(2~{R},4~{S},5~{R},6~{R})-5-acetamido-2-[4-[(2~{R})-3-[2-[(2~{S},3~{R},4~{R},5~{R},6~{R})-6-(hydroxymethyl)-3,4,5-tris(oxidanyl)oxan-2-yl]ethylamino]-3-oxidanylidene-2-(2-phenylethanoylamino)propyl]-1,2,3-triazol-1-yl]-4-oxidanyl-6-[(1~{R},2~{R})-1,2,3-tris(oxidanyl)propyl]oxane-2-carboxylic 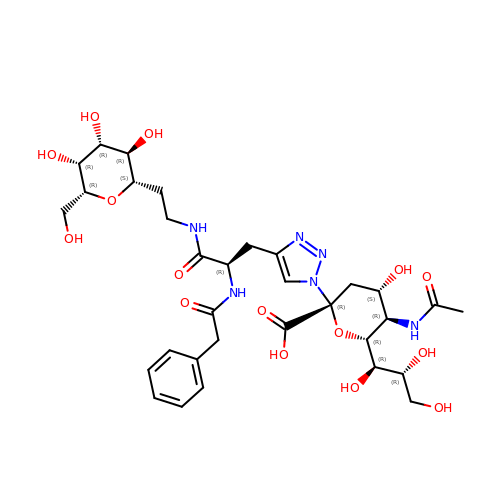acid | C32 H46 N6 O15 | VJJPXKHAIAQVCK-WOQXIOLNSA-N> PNFSGNWKIIRSENFEELLKVLGVNVMLRKIAVAAASKQAVEIKQEGDTFYIKVSTTVYTTEINFKVGEEFEEQTVDGRPCKSLVKWESENKMVCEQKLLKGEGPKTSWTKELTNDGELIET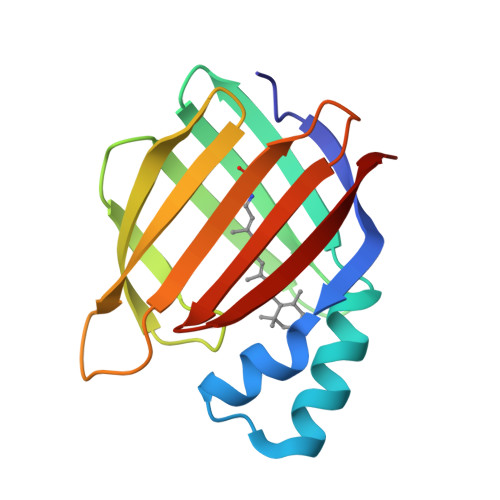MTADDVVCTQVFVRE> GDDLEVGKNIDESAYSGIYENNAYLRDGKSNLVSKVVELHGETYATTVKMGLSKTPNTATSAKVKIDAAYLETYNKAHNTDFALYPQDLVTFANEGILTVNANTKSAEVEMTIRAGEGLQEDKTYAIPVAISDQSSDITIKDEDAKHCIYLVKDMRNAGDAYKGEGVMQGYLFFEVNDVNPLNTLSFQLENGKLLWDVVVLFAANINYDAEAGRPRVQCNPNVQYLLDNNETLLQPLRRRGVKVLLGLLGNHDITGLAQLSEQGAKDFAREVAQYCKAYNLDGVNYDDEYSNSPDLSNPSLTNPSTAAAARLCYETKQAMPDKLVTVFDWGQMYGVATVD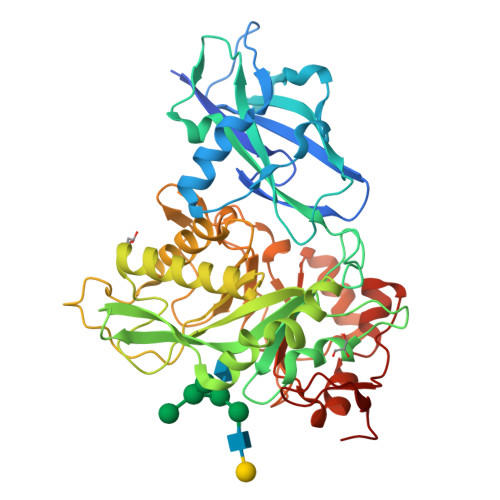GVDAKEWIDIVVANYGSAAYPIGQMTKKQCSGISMEFNLGGGGSLSASKAQSMIDGGYGWFMGFAPSPAKYGSVFSRLQGGGEVLYGSNVAAPTIFYKKNDPTPYKYPDDL> MSTTQTPDLDAIVIGAGFGGIYMLHKLRNDLGLSVRVFEKGGGVGGTWYWNKYPGAKSDTEGFVYRYSFDKELLREYDWTTRYLDQPDVLAYLEHVVERYDLARDIQLNTEVTDAIFD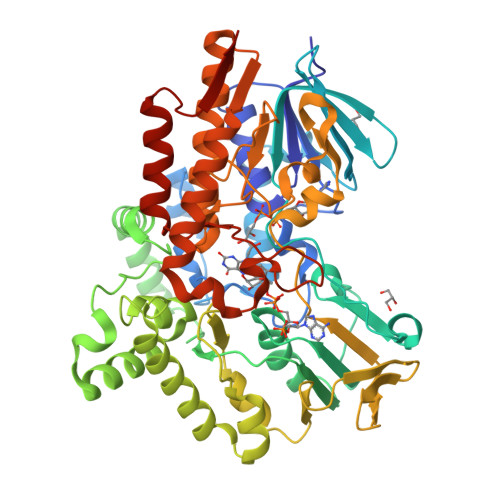EETELWRVTTAGGETLTARFLVTALGLLSRSNIPDIPGRDSFAGRLVHTNAWPEDLDITGKRVGVIGTGSTGTQFIVAAAKMAEQLTVFQRTPQYCVPSGNGPMDPDEVARIKQNFDSIWDQVRSSTVAFGFEESTVEAMSVSESERQRVFQQAWDKGNGFRFMFGTFCDIATNPEANAAAAAFIRSKIAEIVKDPETARKLTPTDLYAKRPLCNEGYYETYNRDNVSLVSLKETPIEEIVPQGVRTSDGVVHELDVLVFATGFDAVDGNYRAMNLRGRDGRHINEHWTEGPTSYLGVTKAGFPNMFMILGPNGPFTNLPPSIEAQVEWISDLIDKATREGLTTVEPTADAEREWTETCAEIANMTLFPKADSWIFGANIPGKRHAVMFYLGGLGNYRRQLADVADGGYRGFQLRGERAQAVA>[2x]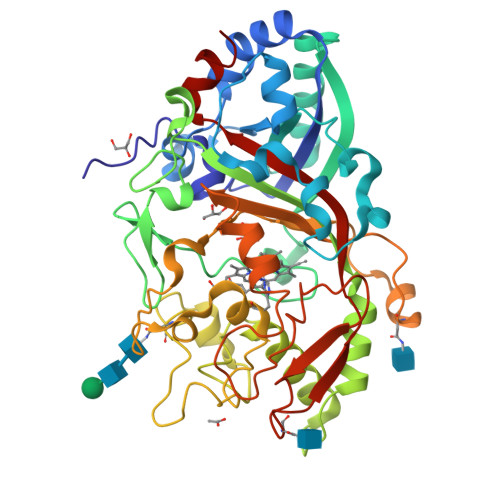ATSLNTDDIQGDILVGMHKQKQLFYFFAINDPATFKTFLASDIAPVVASVTQLSNVATQPLVALNIAFSNTGLLALGVTDNLGDSLFANGQAKDATSFKESTSSWVPQFAGTGIHGVIILASDTTDLIDQQVASIESTFGSSISKLYSLSASIRPGNEAGHEMFGFLDGIAQPAINGFNTPLPGQNIVDAGVIITGATNDPITRPSWAVGGSFLAFRQLEQLVPEFNKYLLDNAPAGSGSLQARADLLGARMVGRWKSGAPIDLTPTADDPALGADAQRNNNFTYSHAGFDLGSDQSHCPFSAHIRKTRPRADLGGSLTPPNLSAGANSIMRSGIPYGPEVTSAESASNTTTQERGLAFVAYQAQLSQGFHFLQQTWADNANFPPGKTPATVGLDPIIGQNNGQPRVVNGLLPSNSSASLSIPQFVVSHGGEYFFSPPISAIGGRLSA> SLPEGKIMPNTVFVGGIDVRM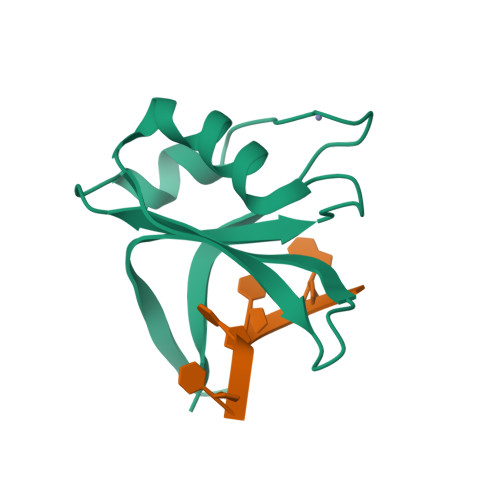DETEIRSFFARYGSVKEVKIITDRTGVSKGYGFVSFYNDVDVQKIVESQINFHGKKLKLGPAIRKQ>[2x]MAYRKRGAR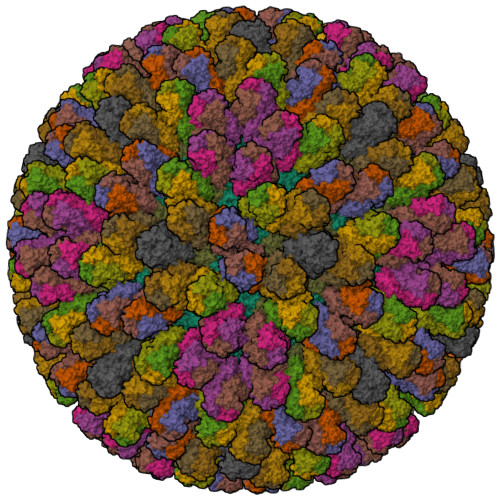REANINNNDRMQEKDDEKQDQNNRMQLSDKVLSKKEEVVTDSQEEIKIADEVKKSTKEESKQLLEVLKTKEEHQKEIQYEILQKTIPTFEPKESILKKLEDIKPEQAKKQTKLFRIFEPRQLPIYRANGEKELRNRWYWKLKKDTLPDGDYDVREYFLNLYDQVLTEMPDYLLLKDMAVENKNSRDAGKVVDSETASICDAIFQDEETEGAVRRFIAEMRQRVQADRNVVNYPSILHPIDYAFNEYFLQHQLVEPLNNDIIFNYIPERIRNDVNYILNMDRNLPSTARYIRPNLLQDRLNLHDNFESLWDTITTSNYILARSVVPDLKELVSTEAQIQKMSQDLQLEALTIQSETQFLTGINSQAANDCFKTLIAAMLSQRTMSLDFVTTNYMSLISGMWLLTVVPNDMFIRESLVACQLAIVNTIIYPAFGMQRMHYRNGDPQTPFQIAEQQIQNFQVANWLHFVNNNQFRQVVIDGVLNQVLNDNIRNGHVINQLMEALMQLSRQQFPTMPVDYKRSIQRGILLLSNRLGQLVDLTRLLAYNYETLMACVTMNMQHVQTLTTEKLQLTSVTSLCMLIGNATVIPSPQTLFHYYNVNVNFHSNYNERINDAVAIITAANRLNLYQKKMKAIVEDFLKRLHIFDVARVPDDQMYRLRDRLRLLPVEVRRLDIFNLILMNMDQIERASDKIAQGVIIAYRDMQLERDEMYGYVNIARNLDGFQQINLEELMRTGDYAQITNMLLNNQPVALVGALPFVTDSSVISLIAKLDATVFAQIVKLRKVDTLKPILYKINSDSNDFYLVANYDWVPTSTTKVYKQVPQQFDFRNSMHMLTSNLTFTVYSDLLAFVSADTVEPINAVAFDNMRIMNEL;>MDVLYSLSKTLKDARDKIVEGTLYSNVSDLIQQFNQMIITMNGNEFQTGGIGNLPIRNWNFDFGLLGTTLLNLDANYVETARNTIDYFVDFVDNVCMDEMVRESQRNGIAPQSDSLRKLSGLKFKRINFDNSSEYIENWNLQNRRQRTGFTFHKPNIFPYSASFTLNRSQPAHDNLMGTMWLNAGSEIQVAGFDYSCAINAPANTQQFEHIVQLRRVLTTATITLLPDAERFSFPRVINSADGATTWYFNPVILRPNNVEVEFLLNGQIINTYQARFGTIIARNFDTIRLSFQLMRPPNMTPAVAALFPNAQPFEHHATVGLTLRIESAVCESVLADASETMLANVTSVRQEYAIPVGPVFPPGMNWTDLITNYSPSREDNLQRVFTVASIRSMLVK[13x]> MKHHHHHHMKQNSPLDEENLTQENQDRGTHVDRGLASANVDFAFSLYKQLVLKAPDKNVIFSPVSISTALAFLSLGAHNTTLTEILKGLKFNLTETSEAEIHQSFQHLLRTLNQSSDELQLSMGNAMFVKEQLSL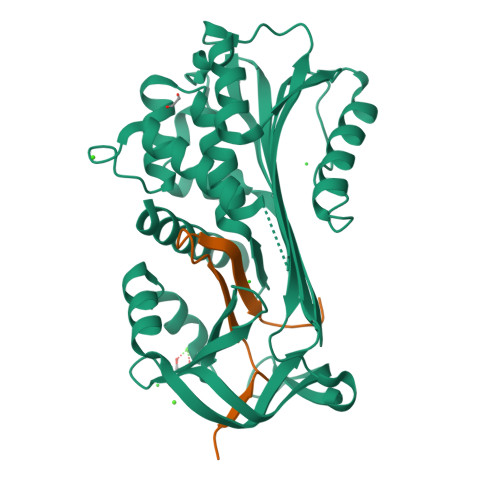LDRFTEDAKRLYGSEAFATDFQDSAAAKKLINDYVKNGTRGKITDLIKDLDSQTMMVLVNYIFFKAKWEMPFDPQDTHQSRFYLSKKKWVMVPMMSLHHLTIPYFRDEELSCTVVQLNYTGNASVFFILPDQDKMEEVEAMLSRETLARWGDSLEFREIGELYLPKFSISRDYNLNDILLQLGIEEAFTSKADLSGITGARNLAVSQVVHKAVLDVFEEGTERSAATAVKITLL;> SALVETRTIVRFNRPFLMIIVDHFTWSIFFMSKVTNPKQA>LFLAQEIIRKKRDGHALSDEEIRFFINGIRDNTISEGQIAALAMTIFFHDMTMPERVSLTMAMRDSGTVLDWKSLHLNGPIVDKHSTGGVGDVTSLMLGPMVAACGGYIPMISGRGLGHTGGTLDKLESIPGFDIFPDDNRFREIIKDVGVAIIGQTSSLAPADKRFYATRDITATVDSIPLITASILAKKLAEGLDALVMDVKVGSGAFMPTYELSEALAEAIVGVANGAGVRTTALLTDMNQVLASSAGNAVEVREAVQFLTGEYRNPRLFDVTMALCVEMLISGKLAKDDAEARAKLQAVLDNGKAAEVFGRMVAAQKGPTDFVENYAKYLPTAMLTKAVYADTEGFVSEMDTRALGMAVVAMGGGRRQASDTIDYSVGFTDMARLGDQVDGQR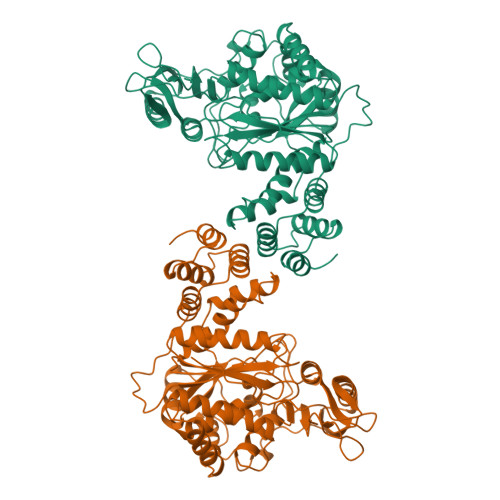PLAVIHAKDENNWQEAAKAVKAAIKLADKAPESTPTVYRRISE[2x]> LKDVNHIHPLPDFVRGGFDYVPSDIFSGKENFEQTLRI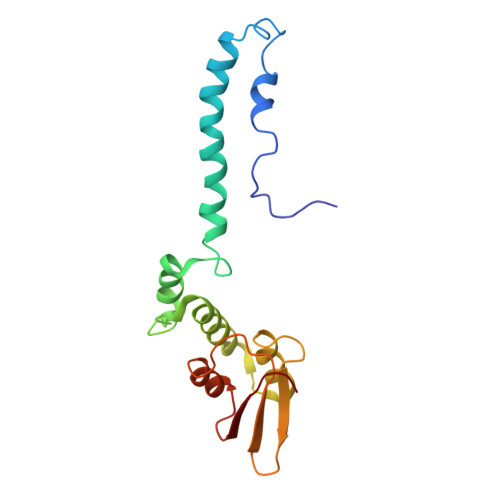LLERLEFIDQKMVELAELRTTLNAEDAILDEIGRQLGIYRNGLNDPEYRAVIMILTGNNSKSGTRADIIATLKQLFGEDGVTTYKGYNYRLDINIFNTCMEVTDILPEIIDMLPLVTHLRVVENQGY>[2x]TPEMPVLENRAAQGDITAPGGARRLTGDQTAALRDSLSDKPAKNIILLIGDGMGDSEITAARNYAEGAGGFFKGIDALPLTGQYTHYALNKKTGKPDYVTDSAASATAWSTGVKTYNGALGVDIHEKDHPTILEMAKAAGLATGNVSTAELQHATPAALVAHVTSRKCYGPSATSEKCPGNALEKGGKGSITEQLLNARADVTLG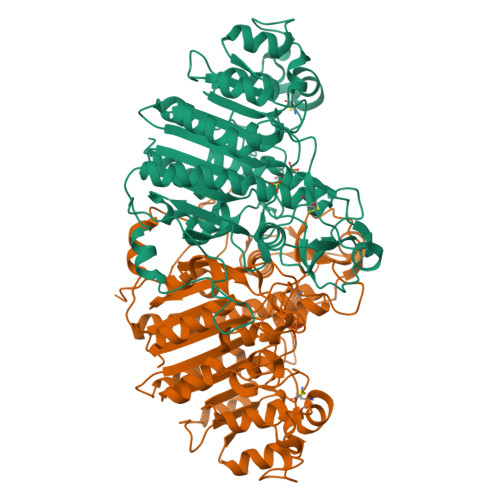GGAKTFAETATAGEWQGKTLREQAQARGYQLVSDAASLNSVTEANQQKPLLGLFADGNMPVRWLGPKATYHGNIDKPAVTCTPNPQRNDSVPTLAQMTDKAIELLSKNEKGFFLQVEGASIDWQDHAANPCGQIGETVDLDEAVQRALEFAKKEGNTLVIVTADHAHASQIVAPDTKAPGLTQALNTKDGAVMVMSYGNSEEDSQEHTGSQLRIAAYGPHAANVVGLTDQTDLFYTMKAALGLK>[4x]MRGSHHHHHHGSMASKVESRQAAVLAIATANPPNIFYQADYPDFYFRVTKSEHMTQLKDKFKRMCEKSMIRKRHMYLTEDVIKENPNIGILNAPSFNARQEIMVEEVPKLGKEAALKAIKEWGQPLSKLTHLIFCTSSGVNMPSADYHLAKIMGLPPYVQRTMIYQQGCFAGATALRLAKDIAENNGGHTRILIVCVELMVVCFQAPSDTYLDLLVG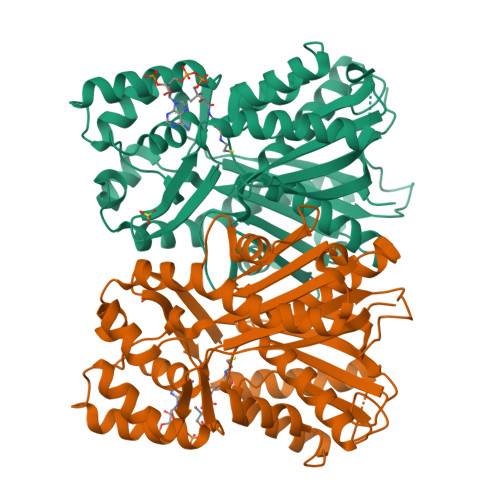NAIFSDGAAAAIVGADLDTTTERPIFNIVSANQTTIPDSEDGIVGHIREMGMKYYLSRTVPQVIGNNIVQCCRDTFTPLGINDWNSMFYIVHPGGPAVLRMMEEKLGLSKERMRASWHVLSEYGNMGGPSVLFILDEMRNKSMEEGKSTTGEGLEWGVMFGFGPGLTVETVVLRSVAIN>MNKPVKKQQPKKVIPNFEYARRLNGKKVKIFLRNGEVLDA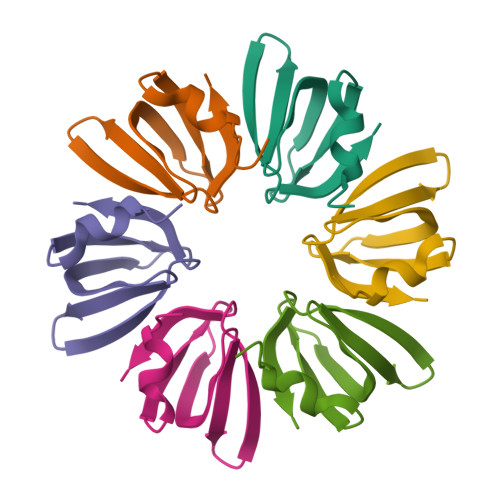EVTGVSNYEIMVKVGDRNLLVFKHAIDYIEY[12x]>SMGIINQVSTVTKVIHHELEVAASADDIWTVYSWPG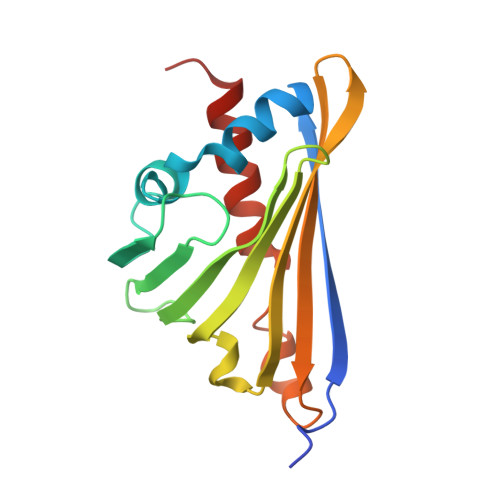LAKHLPDLLPGAFEKLEIIGDGGVGTILDMTFVPGEFPHEYKEKFILVDNEHRLKKVQMIEGGYLDLGVTYYMDTIHVVPTGKDSCVIKSSTEYHVKPEFVKIVEPLITTGPLAAMADAISKLVLEHKS[3x]> MGEPQQVSALPPPPMQYIKEYTDENIQEGLAPKPPPPIKDSYMMFGNQFQCDDLIIRPLESQGIERLHPMQFDHKKELRKLNMSILINFLDLLDILIRSPGSIKREEKLEDLKLLFVHVHHLINEYRPHQARETLRVMMEVQKRQRLETAERFQKHLERVIEMIQNCLASLPDDLPHSEAGMRVKAEPMDTDDNSNCPGQNEQQRESSGHR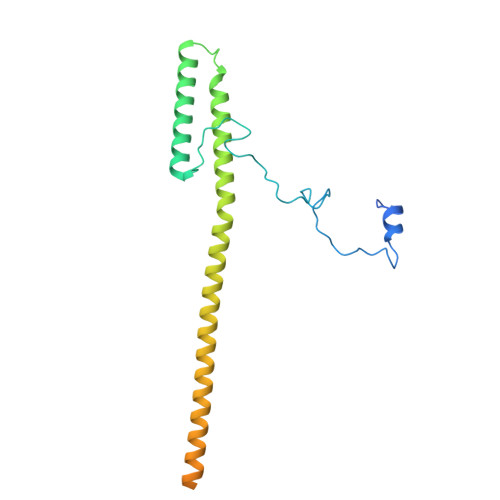RDQIIEKDAALCVLIDEMNERP> MALNFTTITENNVIRDLTTQVNNIGEELTKERNIFDITDDLVYNFNKSQKIKLTDDKGLTKSYGNITALRDIKEPGYYYIGARTLATLLDRPDMESLDVVLHVVPLDTSSKVVQHLYTLSTNNNQIKMLYRFVSGNSSSEWQFIQGLPSNKNAVISGTN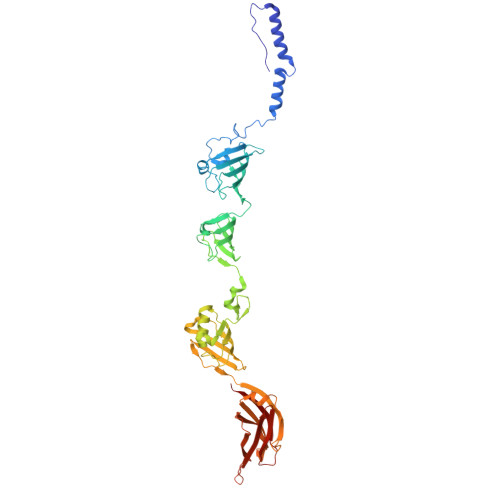ILDIASPGVYFVMGMTGGMPSGVSSGFLDLSVDANDNRLARLTDAETGKEYTSIKKPTGTYTAWKKEFEPKDMEKYLLSSIRDDGSASFPLLVYTSDSKTFQQAIIDHIDRTGQTTFTFYVQGGVSGSPMSNSCRGLFMSDTPNTSSLHGVYNAIGTDGRNVTGSVVGSNWTSPKTSPSHKELWTGAQSFLSTGTTKNLSDDISNYSYVEVYTTHKTTEKTKGNDNTGTICHKFYLDGSGTYVCSGTFVSGDRTDTKPPITEFYRVGVSFKGSTWTLVDSAVQNSKTQYVTRIIGINMP> SGRPSFAGKEYSLEPIDERTPILFQWFEARPERYEKGEVPILNTKEHPYLSNIINAAKIENERIIGVLVDGNFTYEQKKEFLNLENEHQNIAIIYRADVDFSMYDKKLSDIYLENIHKQESYPASERDNYLLGLLREELKNIPEGKDSLIESYAEKREHTWFDFFRNLAILKAGSLFTETGKTGCHNI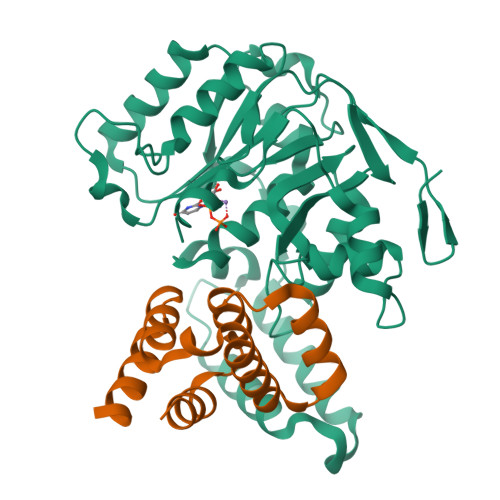SPCSGCIYLDADMIITDKLGVLYAPDGIAVHVDCNDEIKSLENGAIVVNRSNHPALLAGLDIMKSKVDAHPYYDGLGKGIKRHFNYSSLHNYNAFCDFIEFKHENIIPNTSMYTSSSW;> GEEDLCAAFNVICDNVGKDWRRLARQLKVSDTKIDSIEDRYPRNLTERVRESLRIWKNTEKENATVAHLVGALRSCQMNLVADLVQEVQQAR> TV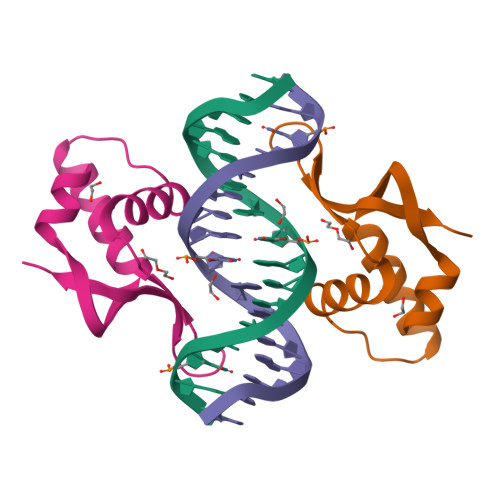QWLLDNYETAEGVSLPRSTLYNHYLLHSQEQKLEPVNAASFGKLIRSVFMGLRTRRLGTRGNSKYHYYGLRIKA>[10x]MPMTDLPSAVTNERTEQTNTTNEQQESKGFDYLIVGAGFAGSVLAERLASSGQRVLIVDRRPHIGGNAYDCYDDAGVLIHPYGPHIFHTNSKDVFEYLSRFTEWRPYQHRVLASVDGQLLPIPINLDTVNRLYGLNLTSFQVEEFFASVAEKVEQVRTSEDVVVSKVGRDLYNKFFRGYTRKQWGLDPSELDASVTARVPTRTNRDNR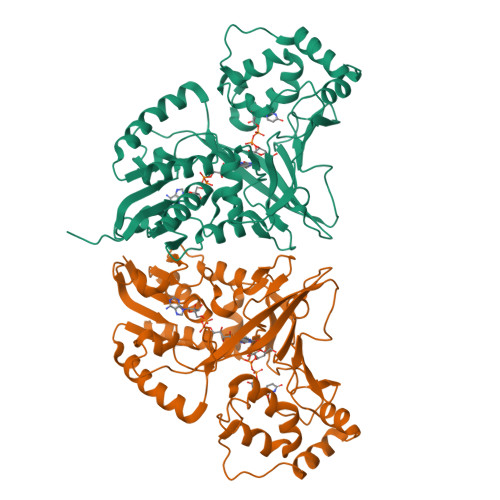YFADTYQAMPLHGYTRMFQNMLSSPNIKVMLNTDYREIADFIPFQHMIYTGPVDAFFDFCYGKLPYRSLEFRHETHDTEQLLPTGTVNYPNDYAYTRVSEFKHITGQRHHQTSVVYEYPRAEGDPYYPVPRPENAELYKKYEALADAAQDVTFVGRLATYRYYNMDQVVAQALATFRRLQGQPEQGNAE> MTRLPKLAVFDLDYTLWPFWVDTHVDPPFHKSSDGTVRDRRGQNIQ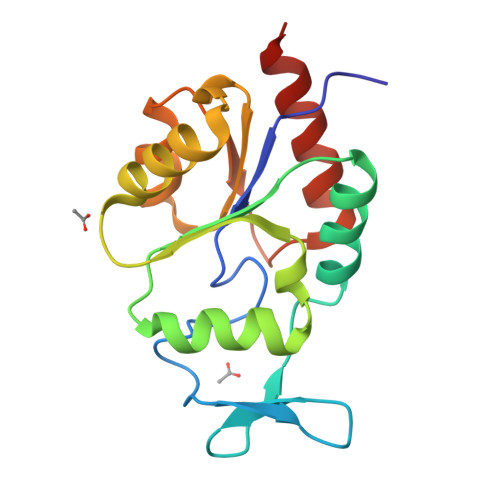LYPEVPEVLGRLQSLGVPVAAASRTSEIQGANQLLELFDLGKYFIQREIYPGSKVTHFERLHHKTGVPFSQMVFFDDENRNIIDVGRLGVTCIHIRDGMSLQTLTQGLETFAKAQAGL> GAMASGKVVKFSYMWTINNFSFCREEMGEVIKSSTFSSGANDKLKWCLRVNPKGLDEESKDYLSLYLLLVSCPKSEVRAKFKFSILNAKGEETKAVESQRAY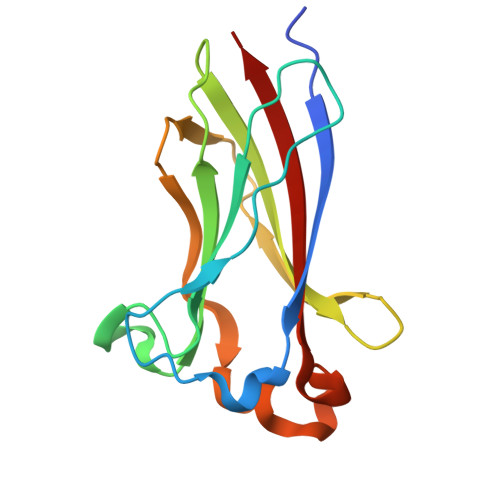RFVQGKDWGFKKFIRRDFLLDEANGLLPDDKLTLFCEVSVVQD>MTDDMLHVMKWHNGEKDYSPFSDAEMTRRQNDVRGWMAKNNVDAALFTSYHCINYYSGWLYCYFGRKYGMVIDHNNATTISAGIDGGQPWRRSFGDNITYTDWRRDNFYRAVRQLTTGAKRIGIEFDHVNLDFRRQLEEALPGVEFVDISQPSMWMRTIKSLEEQKLIREGARVCDVGGAACAAAIKAGVPEHEVAIATTNAMIREIAKSFPFVELMDTWTWFQSGINTDGAHNPVTNRIVQSGDILSLNTFPMIFGYYTALERTLFCDHVDDASLDIWEKNVAVHRRGLELIKPGARCKDIALELNEMYREWDLLKYRSFGYGHSFGVLCHYYGREAGVELREDIDTELKPGMVVSMEPMVMLPEGMPGAGGY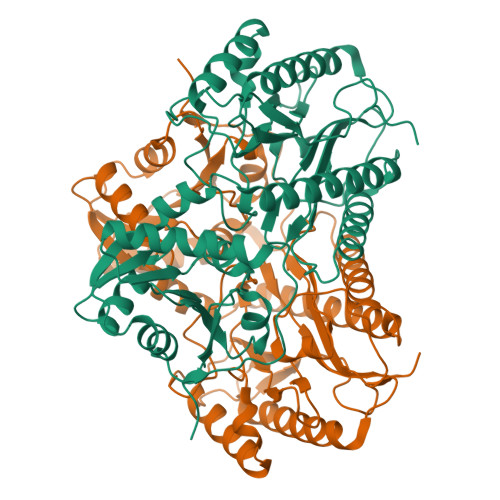REHDILIVGEDGAENITGFPVGPEHNIIRN[6x]> GDVEEAIERAVVHVADTMRSGPSNSASVPALTAVETGHTSQVTPSDTMQTRHVKNYHSRSESTVENFLGRSACVYMEEYKTTDNDVNKKFVAWPINTKQMVQMRRKLEMFTYLRFDMEVTFVITSRQDPGTTLAQDMPVLTHQIMYVPPGGPIPAKVDDYAWQTSTNPSIFWTEGNAPARMSIPFISIGNAYSNFYDGWSNFDQRGSYGYNTLNNLGHIYVRHVSGSSPHPIT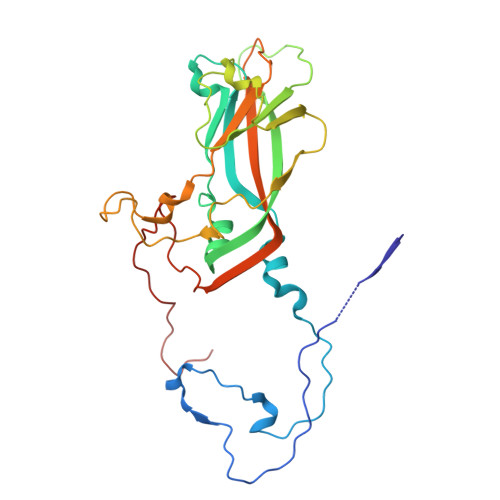STIRVYFKPKHTRAWVPRPPRLCQYKKAFSVDFTPTPITDTRKDINTVT>[8x]GSHMLNRVVLVGRLTKDPELRYTPNG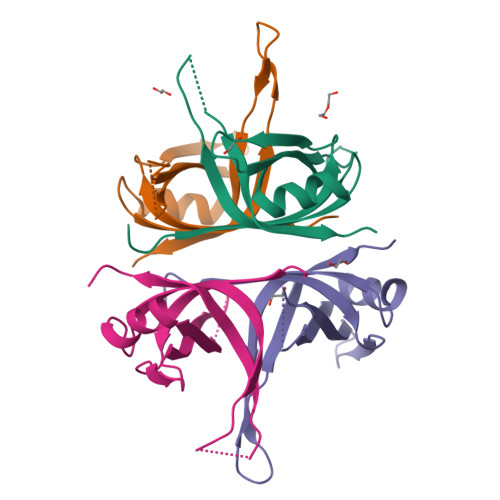AAVATFTLAVNRTFTNQSGEREADFINCVTWRRQAENVANFLKKGSLAGVDGRLQTRNYENQQGQRVFVTEVQAESVQFLEPKNGGGSGSGGY> GAYGAGL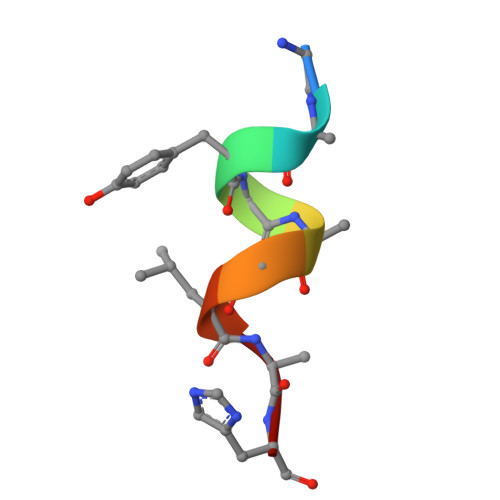AH>PRIDMHSHFFPRISEQEAAKFDANHAPWLQVSA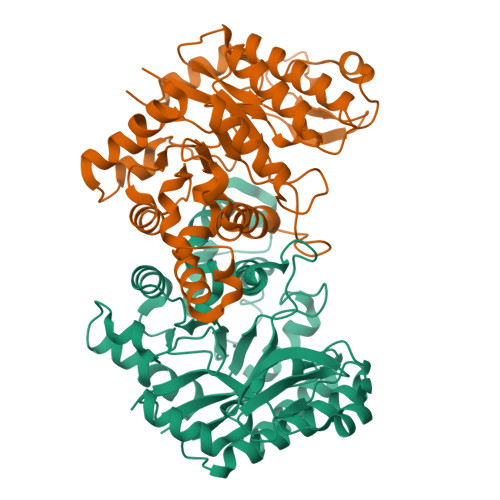KGDTGSIMMGKNNFRPVYQALWDPAFRIEEMDAQGVDVQVTCATPVMFGYTWEANKAAQWAERMNDFALEFAAHNPQRIKVLAQVPLQDLDLACKEASRAVAAGHLGIQIGNHLGDKDLDDATLEAFLTHCANEDIPILVHPWDMMGGQRMKKWMLPWLVAMPAETQLAILSLILSGAFERIPKSLKICFGHGGGSFAFLLGAVDNAWRHRDIVREDCPRPPSEYVDRFFVDSAVFNPGALELLVSVMGEDRVMLGSDYPFPLGEQKIGGLVLSSNLGESAKDKIISGNASKFFNIN[2x]>[2x]METFDPTELPELLKLYYRRLFPYSQYYRWLNYGGVIKNYFQHREFSFTLKDDIYIRYQSFNNQSDLEKEMQKMNPYKIDIGAVYSHRPNQHNTVKLGAFQAQEKELVFDIDMTDYDDVRRCCSSADICPKCWTLMTMAIRIIDRALKEDFGFKHRLWVYSGRRGVHCWVCDESVRKLSSAVRSGIVEYLSLVKGGQDVKKKVHLSEKIHPFIRKSINIIKKYFEEYALVNQDILENKESWDKILALVPETIHDELQQSFQKSHNSLQRWEHLKKVASRYQNNIKNDKYGPWLEWEIMLQYCFPRLDINVSKGINHLLKSPFSVHPKTGRISVPIDLQKVDQFDPFTVPTISFICRELDAISTNEEEKEENEAESDVKHRTRDYKKTSLAPYVKVFEHFLENLDKSRKGELLKKSDLQKDF;>MEFSGRKWRKLRLAGDQRNASYPHCLQFYLQPPSENISLIEFENLAIDRVKLLKSVENLGVSYVKGTEQYQSKLESELRKLKFSYRENLEDEYEPRRRDHISHFILRLAYCQSEELRRWFIQQEMDLLRFRFSILPKDKIQDFLKDSQLQFEAISDEEKTLREQEIVASSPSLSGLKLGFESIYKIPFADALDLFRGRKVYLEDGFAYVPLKDIVAIILNEFRAKLSKALALTARSLPAVQSDERLQPLLNHLSHSYTGQDYSTQGNVGKISLDQIDLLSTKSFPPCMRQLHKALRENHHLRHGGRMQYGLFLKGIGLTLEQALQFWKQEFIKGKMDPDKFDKGYSYNIRHSFGKEGKRTDYTPFSCLKIILSNPPSQGDYHGCPFRHSDPELLKQKLQSYKISPGGISQILDLVKGTHYQVACQKYFEMIHNVDDCGFSLNHPNQFFCESQRILNGGKDIKKEPIQPETPQPKPSVQKTKDASSALASLNSSLEMDMEGLEDYFSEDS[2x];>ADEEQVFHFYWLDAYEDQYNQPGVVFLFGKVWIESAETHVSCCVMVKNIERTLYFLPREMKIDLNTGKETGTPISMKDVYEEFDEKIATKYKIMKFKSKPVEKNYAFEIPDVPEKSEYLEVKYSAEMPQLPQDLKGETFSHVFGTNTSSLELFLMNRKIKGPCWLEVKSPQLLNQPVSWCKAEAMALKPDLVNVIKDVSPPPLVVMAFSMKTMQNAKNHQNEIIAMAALVHHSFALDKAAPKPPFQSHFCVVSKPKDCIFPYAFKEVIEKKNVKVEVAATERTLLGFFLAKVHKIDPDIIVGHNIYGFELEVLLQRINVCKAPHWSKIGRLKRSNMPKLGGRSGFGERNATCGRMICDVEISAKELIRCKSYHLSELVQQILKTERVVIPMENIQNMYSESSQLLYLLEHTWKDAKFILQIMCELNVLPLALQITNIAGNIMSRTLMGGRSERNEFLLLHAFYENNYIVPDKQIFRKPQQKLGDEDEEIDGDTNKYKKGRKKAAYAGGLVLDPKVGFYDKFILLLDFNSLYPSIIQEFNICFTTVQRVASEAQKVTEDGEQEQIPELPDPSLEMGILPREIRKLVERRKQVKQLMKQQDLNPDLILQYDIRQKALKLTANSMYGCLGFSYSRFYAKPLAALVTYKGREILMHTKEMVQKMNLEVIYGDTDSIMINTNSTNLEEVFKLGNKVKSEVNKLYKLLEIDIDGVFKSLLLLKKKKYAALVVEPTSDGNYVTKQELKGLDIVRRDWCDLAKDTGNFVIGQILSDQSRDTIVENIQKRLIEIGENVLNGSVPVSQFEINKALTKDPQDYPDKKSLPHVHVALWINSQGGRKVKAGDTVSYVICQDGSNLTASQRAYAPEQLQKQDNLTIDTQYYLAQQIHPVVARICEPIDGIDAVLIATWLGLDPTQFRVHHYHKDEENDALLGGPAQLTDE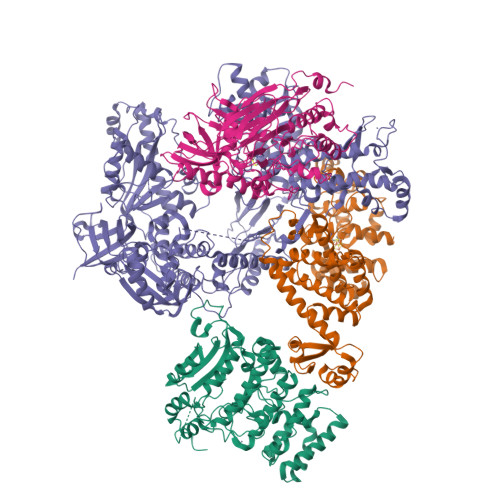EKYRDCERFKCPCPTCGTENIYDNVFDGSGTDMEPSLYRCSNIDCKASPLTFTVQLSNKLIMDIRRFIKKYYDGWLICEEPTCRNRTRHLPLQFSRTGPLCPACMKATLQPEYSDKSLYTQLCFYRYIFDAECALEKLTTDHEKDKLKKQFFTPKVLQDYRKLKNTAEQFLSRSGYSEVNLSKLFAGCAVKS[2x];>[2x]SASAQQLAEELQIFGLDCEEALIEKLVELCVQYGQNEEGMVGELIAFCTSTHKVGLTSEILNSFEHEFLSKRLSKARHSTCKDSGHAGARDIVSIQELIEVEEEEEILLNSYTTPSKGSQKRAISTPETPLTKRSVSTRSPHQLLSPSSFSPSATPSQKYNSRSNRGEVVTSFGLAQGVSWSGRGGAGNISLKVLGCPEALTGSYKSMFQKLPDIREVLTCKIEELGSELKEHYKIEAFTPLLAPAQEPVTLLGQIGCDSNGKLNNKSVILEGDREHSSGAQIPVDLSELKEYSLFPGQVVIMEGINTTGRKLVATKLYEGVPLPFYQPTEEDADFEQSMVLVACGPYTTSDSITYDPLLDLIAVINHDRPDVCILFGPFLDAKHEQVENCLLTSPFEDIFKQCLRTIIEGTRSSGSHLVFVPSLRDVHHEPVYPQPPFSYSDLSREDKKQVQFVSEPCSLSINGVIFGLTSTDLLFHLGAEEISSSSGTSDRFSRILKHILTQRSYYPLYPPQEDMAIDYESFYVYAQLPVTPDVLIIPSELRYFVKDVLGCVCVNPGRLTKGQVGGTFARLYLRRPAADGAERQSPCIAVQVVRI> IESIIKTATDTVKSEINAELGVVPSLNAVETGATSNTEPEEAIQTRTVINQHGVSETLVENFLSRAALVSKRSFEYKDHTSSTARADKNFFKWTINTRSFVQLRRKLELFTYLRFDAEITILTTVAVNGSGNNTYVGL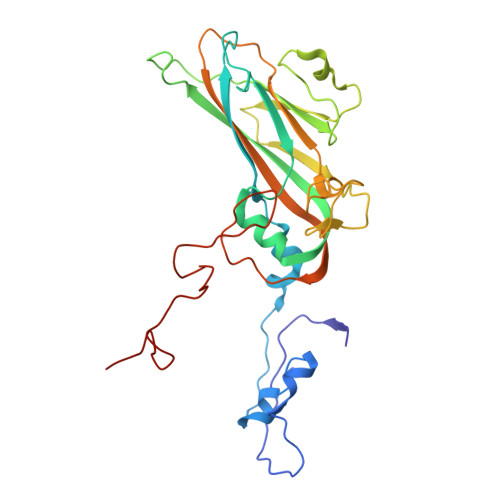PDLTLQAMFVPTGALTPEKQDSFHWQSGSNASVFFKISDPPARITIPFMCINSAYSVFYDGFAGFEKNGLYGINPADTIGNLCVRIVNEHQPVGFTVTVRVYMKPKHIKAWAPRPPRTLPYMSIANANYKGKERAPNALSAIIGNRDSVKTMPHNIVN1-(2,5-dimethylfuran-3-yl)methanamine 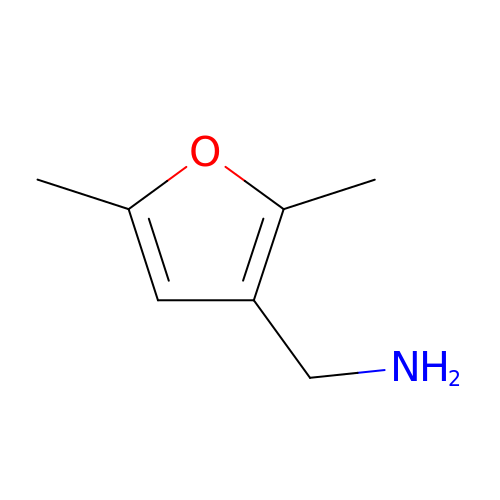| C7 H11 N O | AGQXLVABIKZJJG-UHFFFAOYSA-N>CUUGCUGAGGUGCACACAGCAA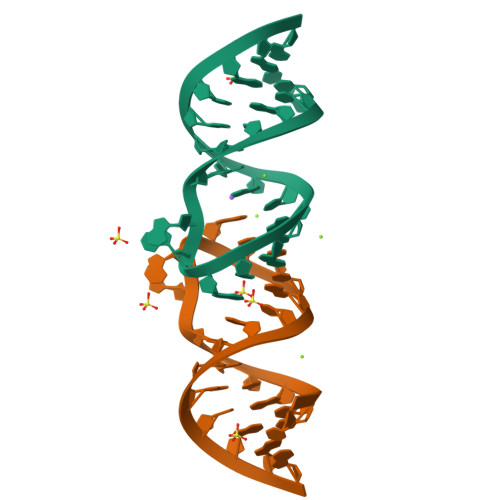G[2x]>[5x]MTDMNILDLFLKASLLVKLIMLILIGFSIASWAIIIQRTRILNAAAREAEAFEDKFWSGIELSRLYQESQGKRDNLTGSEQIFYSGFKEFVRLHRANSHAPEAVVEGASRAMRISMNRELENLETHIPFLGTVGSISPYIGLFGTVWGIMHAFIALGAVKQATLQMVAPGIAEALIATAIGLFAAIPAVMAYNRLNQRVNKLELNYDNFMEEFTAILHRQAFTVSESNKG;>MARARGRGRRDLKSEINIVPLLDVLLVLLLIFMATAPIITQSVEVDLPDATESQAVSSNDNPPVIVEVSGIGQYTVVVEKDRLERLPPEQVVAEVSSRFKAN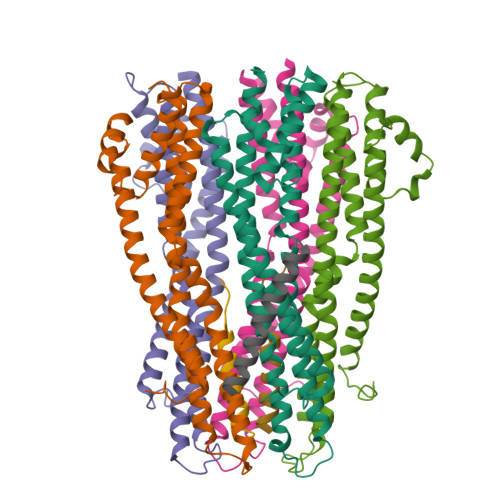PKTVFLIGGAKDVPYDEIIKALNLLHSAGVKSVGLMTQPILEHHHHHHHH[2x];> MSKATEQNDKLKRAIIISAVLHVILFAALIWSSFDENIEASAGGGGGSSIDAVMVDSGAVVEQYKRMQSQESSAKRSDEQRKMKEQQAAEELREKQAAEQERLKQLEKERLAAQEQKKQAEEAAKQAELKQKQAEEAAAKAAADAKAKAEADAKAAEEAAKKAAADAKKKAEAEAAKAAAEAQKKAEAAAAALKKKAEAAEAAAAEARKKAATEAAEKAKAEAEKKAAAEKAAADKKAAAEKAAADKKAAEKAAAEKAAADKKAAAEKAAADKKAAAAKAAAEKAAAAKAAAEADDIFGELSSGKNAPKTGGGAKGNNASPAGSGNTKNNGASGADINNYAGQIKSAIESKFYDASSYAGKTCTLRIKLAPDGMLLDIKPEGGDPALCQAALAAAKLAKIPKPPSQAVYEVFKNAPLDFKP>[6x]SMSPEPDCQKQFQAAVSVIQNLPKNGSYRPS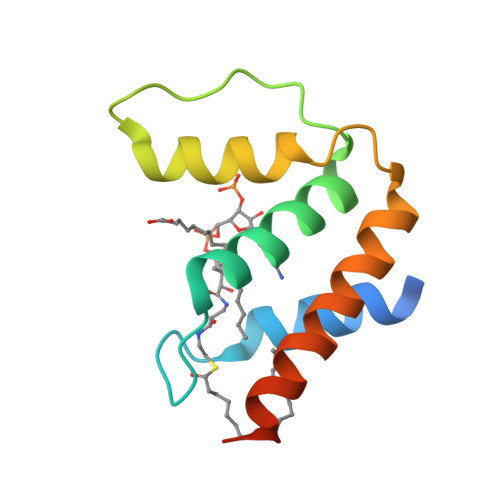YEEMLRFYSYYKQATMGPCLVPRPGFWDPIGRYKWDAWNSLGKMSREEAMSAYITEMKLVAQKVIDTVPLGEVAE> MVQRIYLDNNATTRIDPKVKEIMDPFLRDHYGNPSSLHQFGTETHPAIAEALDKLYKGINARDIDDVIITSCATESNNWVLKGVYFDECLKKGKNHIVTTVAEHPAVRSTCNFLESLGVEVTYLPINEHGSITAEQVREAITEKTALVSVMWANNETGLIFPIEEIGAICKEKGVLFHTDAVQAIGKIPVDVLKANAD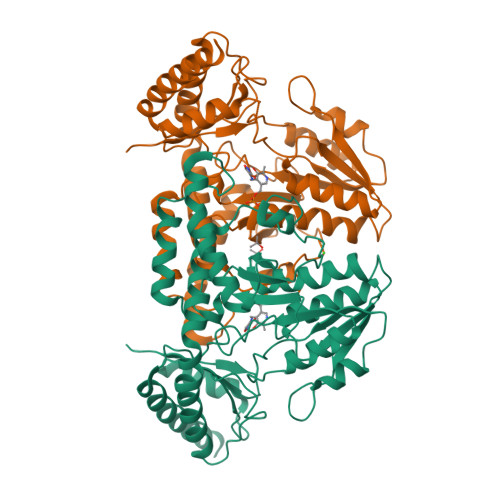FLSFSAHKFHGPKGIGGLYIRSGVGLTPLFHGGEHMNGRRSGTLNVPYIVGMGEAMKLAVEHLDYEKEVVGKLRDKLEEALLKIPDVMVVGDRIHRVPNTTLVSVRGIEGEAMLWDLNRSNIAASTGSACASEDLEANPVMVAIGASKELAHTAIRLSLSRFNTEAEIDKTIEVFSQAAVRLRNISSSYVDLVPRGSHHHHHH>VEFDRADILYNIRQTSRPD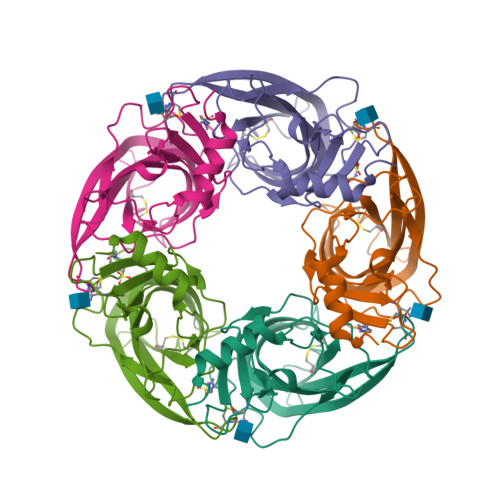VIPTQRDRPVAVSVSLKFINILEVNEITNEVDVVFWQQTTWSDRTLAWNSSHSPDQVSVPISSLWVPDLAAYNAISKPEVLTPQLARVVSDGEVLYMPSIRQRFSCDVSGVDTESGATCRIKIGSWTHHSREISVDPTTENSDDSEYFSQYSRFEILDVTQKKNSVTYSCCPEAYEDVEVSLNFRKKGRSEIL[10x]>MKMKLAVLPGDGIGPEVMDAAIRVLKTVLDNDGHEAVFENALIGGAAIDEAGTPLPEETLDICRRSDAILLGAVGGPKWDHNPASLRPEKGLLGLRKEMGLFANLRPVKAYATLLNASPLKRERVENVDLVIVRELTGGLYFGRPSERRGPGENEVVDTLAYTREEIERIIEKAFQLAQIRRKKLASVDKANVLESSRMWREIAEETAKKYPDVELSHMLVDSTAMQLIANPGQFDVIVTENMFGDILSDLASVI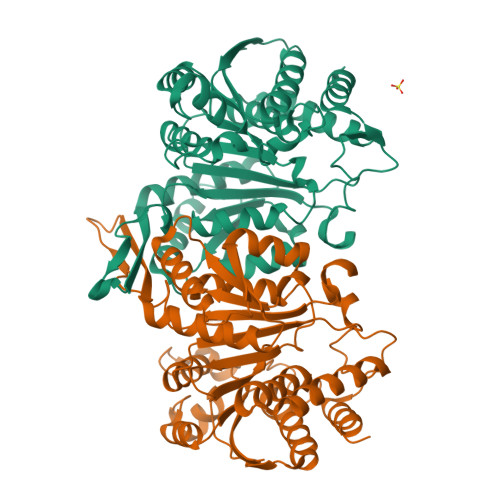TGSLGMLPSASLRSDRFGMYEPVHGSAPDIAGQGKANPLGTVLSAALMLRYSFGLEKEAAAIEKAVDDVLQDGYCTGDLQVANGKVVSTIELTDRLIEKLNNSAAGPRIFQ[8x]> MVAKGRIIRVTGPLVVADGMKGAKMYEVVRVGELGLIGEIIRLEGDKAVIQVYEETAGVRPGEPVVGTGASLSVELGPGLLTSIYDGIQRPLEVIREKTGDFIARGVTAPALPRDKKWHFIPKAKVGDKVVGGDIIGEVPETSIIVHKIMVPPGIEGEIVEIAEEGDYTIEEVIAKVKTPSGEIKELKMYQRWPVRVKRPYKEKLPPEVPLITGQRVIDTFFPQAKGGTAAIPGPFGSGKTVTQHQLAKWSDAQVVIYIGCGERGNEMTDVLEEFPKLKDPKTGKPLMERTVLIANTSNMPVAAREASIYTGITIAEYFRDMGYDVALMADSTSRWAEALREISGRLEEMPGEEGYPAYLASKLAEFYERAGRVVTLGSDYRVGSVSVIGAVSPPGGDFSEPVVQNTLRVVKVFWALDADLARRRHFPAINWLTSYSLYVDAVKDWWHKNIDPEWKAMRDKA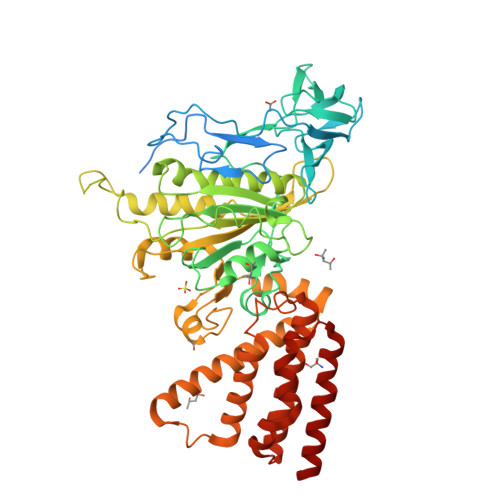MALLQKESELQEIVRIVGPDALPERERAILLVARMLREDYLQQDAWDEVDTYCPPEKQVTMMRVLLNFYDKTMEAINRGVPLEEIAKLPVREEIGRMKFERDVSKIRSLIDKTNEQFEELFKKYGA>[3x]MSNSNVETFFKSSSEKNKNNFKEISCCFKISNEERSLPFQLIWSGIIIISCIGMFWNVVENIKLYFYSSPSVKFEYIKNDSLYFPAITICPFLLNWNPFFTESISFFPEMNDIFEIIETNEYDMLYLWNKTDEYFQYDDSYVYQDALIEEDEFDRSSIIPNTEIMSVSGKCHMYSLEEPVYIGNAIPNILIVYNHSKIYKDKWIKVLIHSIEDKLTSHFFAINVGVDSLLQQMTEVNFQVIQKINLNLSNNPCLFPEEVDKCFKKCLDNFMFKDLSRIHKCRLPFMDYPPDIPYCNYTNFPQMYTRFNKILKGFNKTNCLCPRKCRETRYEIQYQFNIGGFNNQTFIKITSRNSITLETEYWSYNFYSLLSDIGGSLGLFLGASILSMCEIMQKILRNFCMYSLSLKNRVLSRNSVHKINY

In this study, we identified a proton-dissociation-permeated sodium channel (PDPNaC1) in the antennal sensory neurons of the centipede Scolopendra subspinipes mutilans. PDPNaC1, which is permeable to monovalent cations, assembles as a homotrimer. Unlike most proton-gated channels, where proton binding induces currents, PDPNaC1’s transient ion-permeable state is triggered by proton dissociation. Thus, the identification of PDPNaC1 suggests the remarkable diversity of proton responses and molecular mechanisms in DEG/ENaC family.

At pH 8.0, approximately 121,831 selected particles yielded an EM reconstruction at an overall resolution of 3.03 Å. The architecture of PDPNaC1 is composed of three homologous subunits, each featuring two transmembrane (TM) helices. The extracellular domain of each PDPNaC1 subunit, containing 12 β-strands and 6 α-helices, forms the palm, thumb, finger, and β-ball regions, which are common features among DEG/ENaC family members. Notably, despite sharing these conserved structural features, PDPNaC1 lacks the extracellular knuckle domain, which mediates proton-induced activation and desensitization rearrangements in cASIC1a. To identify the potential proton-sensor, we calculated the protein charge distribution of PDPNaC1 (at pH 8.0) and identified a negatively charged cavity near the extracellular domain apex, formed by residues D227, D145, and Y143 in the β-ball and palm domains. The pore radius profile corresponds to the non-conductive state observed in PDPNaC1 at pH 8.0. Along the ion pathway, we observed two constriction sites corresponding to residues Asp372 and Gly375 with pore radii of 0.86 Å and 0.39 Å, respectively. These distances are insufficient to accommodate a sodium ion (radius 1.02 Å), thereby constituting two gates (upper and lower) within the central pathway, analogous to those observed at Asp433 and Gly436 in the cASIC1a channel. Above the Gly-Ala-Ser motif, we identified a narrow constriction site where Gly378 from each subunit converges to form a hydrophobic seal, with a pore radius of 1.28 Å. Notably, substitution at position 378 (mutants Gly378Ser and Gly378Gln) significantly altered ion selectivity, reducing the permeability ratios of monovalent cations to Na+, especially for Cs+, indicating that the mutants enhance selectivity for Na+. These results suggest that Gly378 contributes to maintaining a permissive pore constriction, thereby enabling broader ion permeability in the wild-type channel.The dual-functional transporters, called ABC-transporter maturation and secretion (AMS) proteins or peptidase-containing ATP-binding transporters (PCAT), excise a leader sequence concomitant with the unidirectional extracellular export of the mature peptide. Following the installation of these posttranslational modifications, the cognate AMS/PCAT catalyzes the removal of the leader peptide via cleavage at the double Gly motif and extracellular secretion of the bioactive natural product. Here, we identified and characterized LahT150, a sequence tolerant protease domain of the full-length AMS/PCAT LahT. We show that this protease can remove leader peptides from a large number of double Gly motif-containing peptides.

We therefore synthesized peptide 1 representing the C-terminal 13 amino acids of the ProcA2.8 leader peptide with an aldehyde in the terminal position. A shorter construct, including residues 1–147 (hereafter LahT147; as identified by secondary structure analysis) and a TEV cleavable His6-tag, was used for crystallography. Incubation of peptide 1 with LahT147 prior to crystallization yielded crystals of the binary complex that diffracted to 2.0 Å resolution. The crystallographic asymmetric unit contains four copies of the complex allowing for multiple independent and unbiased views of the protein-peptide complex structure. The overall structure of LahT147 recapitulates the α/β fold observed in the structures of other papain-like peptidase C39 members, wherein a central six-stranded antiparallel β-sheet is surrounded by five α-helices that pack on either side. The catalytic triad of LahT147 is interspersed among the secondary structural elements, with His101 and Asp117 situated on strands β4 and β5, respectively, and the nucleophilic Cys27 on helix α1, which borders one side of the central sheet assembly. Clear and continuous density corresponding to the peptide aldehyde 1 can be observed bound covalently to Cys27 as a thiohemiacetal in all four crystallographically independent molecules. The peptide binds in a groove formed between helices α1–α3 and the central antiparallel β-sheet. The C-terminus of peptide 1, which consists of residues Gly−1 through Ala−3 that correspond to the P1 through P3 positions of the precursor substrate (per the nomenclature of Schechter and Berger [Schechter and Berger, 1967]) binds in a linear manner to the corresponding protease subsites. In contrast, residues Val−4 through Ser−11 form a short two-turn helix, which positions residues Val−4, Leu−7, and Leu−12 of the leader peptide into a hydrophobic groove in LahT150, located roughly 20 Å away from the active site.

>MSKKQIQPVTRGRAKVPVIMQMEALECGAASLAMVLAYYKKWVPLEQVRVDCGVSRDGSNALNVLKAARNYGLEAKGYRYEPEKLKKEGTFPCIIHWNFNHFVVLKGFKGKYAYINDPAKGDVKIPMEEFDRSFTGICLIFKPTDRF[4x];>[4x]GNLSDDELEGVAGG> GSHMETAKEPCMAKFGPLPSK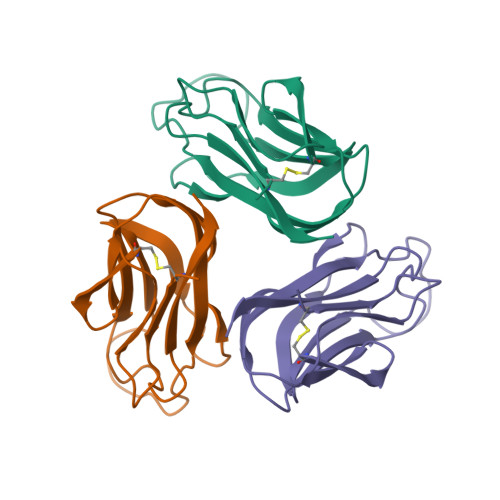WQMASSEPPCVNKVSDWKLEILQNGLYLIYGQVAPNANYNDVAPFEVRLYKNKDMIQTLTNKSKIQNVGGTYELHVGDTIDLIFNSEHQVLKNNTYWGIILLANPQFIS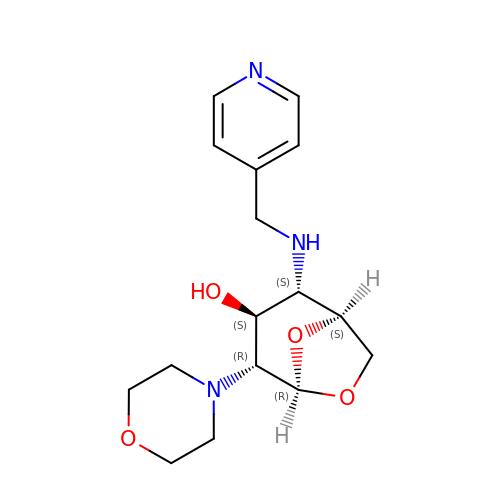(1S,2S,3S,4R,5R)-4-(morpholin-4-yl)-2-[(pyridin-4-ylmethyl)amino]-6,8-dioxabicyclo[3.2.1]octan-3-ol | C16 H23 N3 O4 | RCXMXLJCXLGFHQ-DGXTUMSLSA-N>SLVTTMCLLANVTFPCAQPPICYDRKPAETLAMLSVNV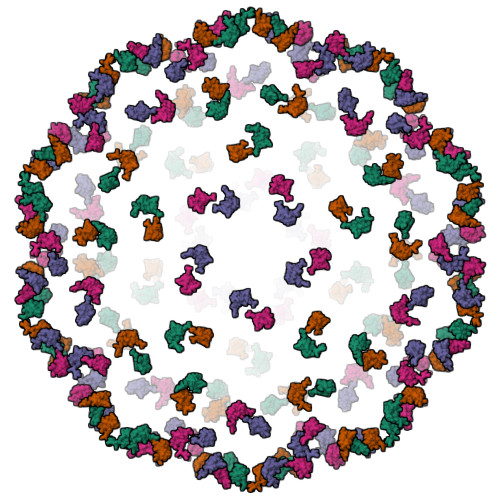DNPGYDELLEAAVKCPGRKRR[4x]> GPHMRWYPWLRPDFEKLVASYQAGRGHHALLIQALPGMGDDALIYALSRYLLCQQ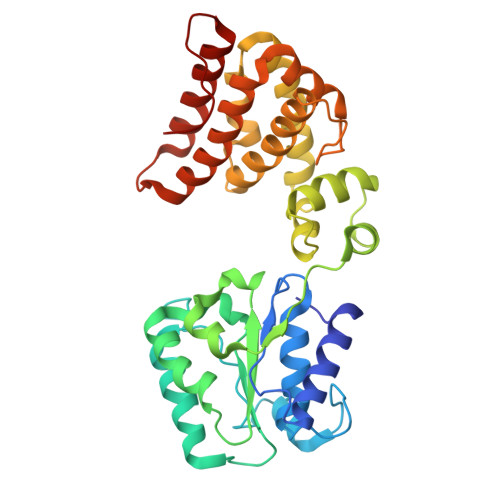PQGHKSCGHCRGCQLMQAGTHPDYYTLAPEKGKNTLGVDAVREVTEKLNEHARLGGAKVVWVTDAALLTDAAANALLKTLEEPPAETWFFLATREPERLLATLRSRCRLHYLAPPPEQYAVTWLSREVTMSQDALLAALRLSAGSPGAALALFQGDNWQARETLCQALAYSVPSGDWYSLLAALNHEQAPARLHWLATLLMDALKRHHGAAQVTNVDVPGLVAELANHLSPSRLQAILGDVCHIREQLMSVTGINRELLITDLLLRIEHYLQPGVVLPVPHL METHYL(2-ACETOXY-2-(2-CARBOXY-4-AMINO-PHENYL))ACETATE 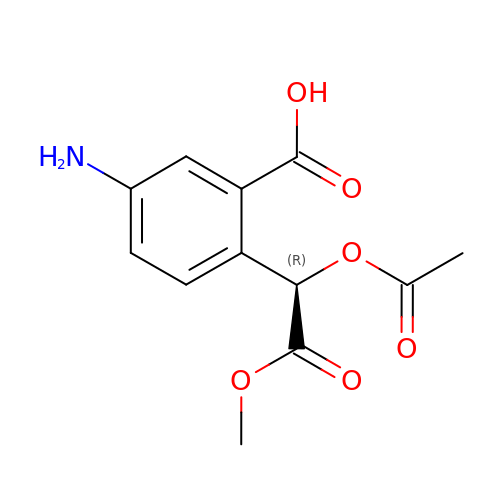| C12 H13 N O6 | DWYLZBJDRMVVPU-SNVBAGLBSA-N> MMSVQKANTVSRQKATGAHFTPDKLAEVIAKRILDYFKGEKNRVIRVLDPACGDGELLLAINKVAQSMNIQLELIGVDFDIDAINIANERLSRSGHKNFRLINKDFLEMVSEGDNYDLFNIEELEPVDIIIANPPYVRTQILGAEKAQKLREKFNLKGRVDLYQAFLVAMTQQLKSNGIIGVITSNRYLTTKGGESTRKFLVSNFNILEIMDLGDSKFFEAAVLPAIFFGEKKNKEYQKENSNVPKFFKIYEQSDIEASSSVNSEFNSLIELLEVNKSGLYSVEDKTYSIS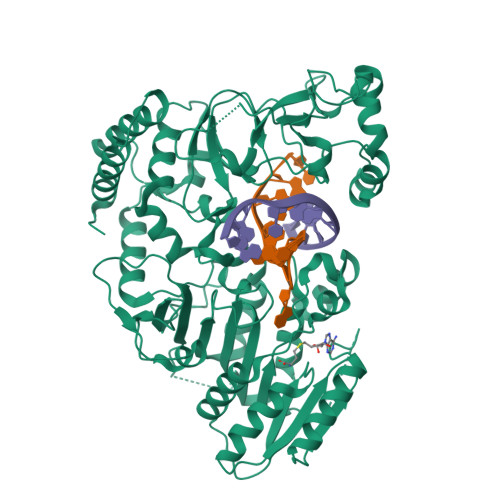LGKIISPENYKEPWILATEDEYEWFMKVNQNAYGFIEDFAHVKVGIKTTADSVFIRSDWGELPEEQIPEDKLLRPIISADQANKWSVSLVGNNKKVLYTHEIRDGQIKAINLEEFPRAKNYLESHKERLASRKYVLKANRNWYEIWVPHDPSLWDKPKIIFPDTSPEPKFFYEDKGSVVDGNCYWIIPKKENSNDILFLIMGICNSKFMSKYHDIAFQNKLYAGRRRYLTQYVNKYPIPDPESIYSKEIISLVRELVNNKKETQDINEIENRIEKLILRAFDIESLKYHHHHHH> GFPTELKPGTNQFLTTDD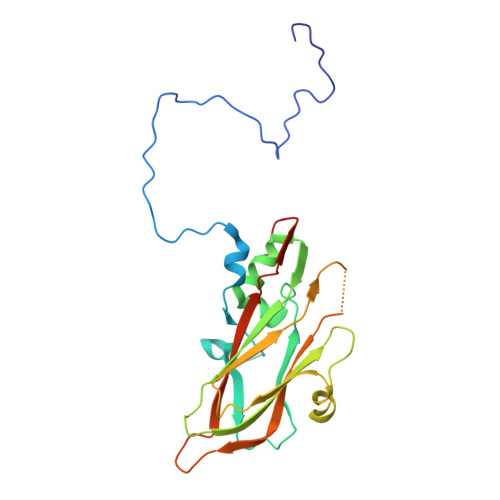GTSPPILPGFEPTPLIHIPGEFTSLLDLCQVETILEVNNTTGTTGVSRLLIPVRAQNNVDQLCASFQVDPGRNGPWQSTMVGQICRYYTQWSGSLKVTFMFTGSFMATGKMLIAYTPPGSAQPTTREAAMLGTHIVWDFGLQSSVTLVIPWISNTHFRAVKTGGVYDYYATGIVTIWYQTNFVVPPDTPTEANIIALGAAQKNFTLKLCKDTDEIQQTAEYQ> MKQLSVSLAILCAVATSEAFAADELQQRAQGLFKPVPAKAPTLKGNPASPVKVELGKMLYFDPRLSASHLISCNTCHNVGLGGGDLQATSTGHKWQQGPINAPTVLNSVFNTAQFWDGRAK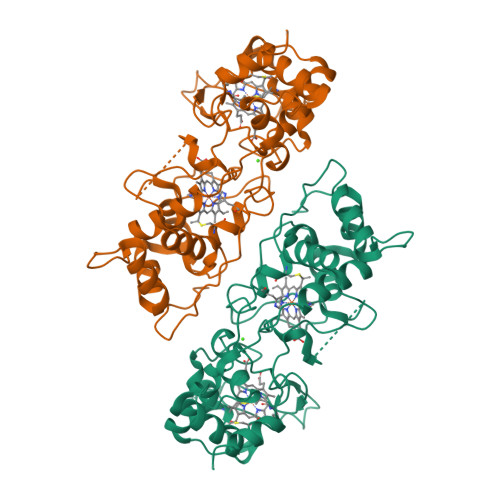DLAEQAKGPVQASVEMNNTPDQVVKTLNSIPDYVALFKKAFPGEKDPVTFDNMAKAIEVFEATLITPDSPFDQYLKGKKKALDGKQTAGLKLFLDKGCVACHGGLNLGGTGYFPFGVVEKPAENILPLGDKGRFAVTNTAKDEYVFRAPSLRNVAITYPYFHSGVVWSLKEAVAVMGSAQFGIKLSDDESEAIAAFLGSLTGKQPKVVYPIMPASTDATPRPRL> QIPASEQETLVRPKPLLLKLLKSVGAQKDTYTMKEVLFY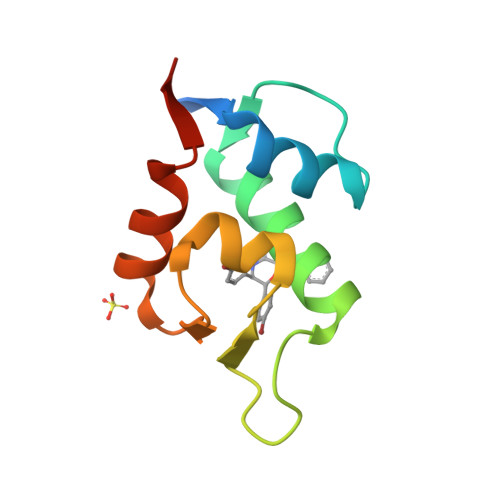LGQYIMTKRLYDEKQQHIVYCSNDLLGDLFGVPSFSVKEHRKIYTMIYRNLVVVNGS>GSHMESFLLSKVSFVIKKIRLEKGMTQEDLAYKSNLDRTAISGIERNSRNLTIKSLELIMKGLEVSDVVFFEMLIKEILKHD[2x]

The most widespread of these mechanisms employs a “controller” (C) protein encoded by a gene downstream of its own promoter, and usually co-transcribed with the endonuclease (R) gene as a single transcriptional unit. The C-protein binds at various sites within the C/R promoter to regulate transcription of its own gene and the associated endonuclease gene. Unusually, in the RM system Esp1396I, the C-protein also represses the MTase (M) gene by binding to the promoter at the transcriptional start site, denoted OM where the C/R genes and the M gene are transcribed convergently from different promoters. Flexibility in this loop is very important for DNA sequence recognition, as it has been observed in the nucleoprotein structures to adopt different conformations depending on which operator site the protein is bound to.

The Y37A and Y37F mutants had KDs that were 11 and 3.5 fold higher than the wild type respectively. The three-fold difference between these two mutants indicates that both the phenyl ring and the hydroxyl group of the tyrosine are important for interacting with the DNA. SPR analysis showed that Y37F formed much more stable complexes with the OM operator site than Y37A, with KDs of 1.8 and 5.5 nM respectively, but both were less stable than the wild type (KD = 0.51 nM). This indicated that the role of the tyrosine was more than just the formation of a hydrogen bond with the DNA backbone, but also involved the phenyl ring common to both tyrosine and phenylalanine. The free protein structures of the wild type, Y37F and Y37A mutants showed no major structural differences either in the local binding regions in terms of helix or side chain positions, or in the overall fold. The ΔΔG for the phenyl group alone (comparing the values for Y37F and Y37A), is −2.8 kJ mol−1 (−1.4 kJ mol−1 per monomer). In terms of crystal packing interactions, the Y37A crystal structure is identical to the triclinic wild type structure but adopts loop conformation I in both monomers in the asymmetric unit. The SO4 based interaction observed in the high-resolution wild type structure is also observed in the Y37A, S52A and monoclinic R46A structures.> AEQATKSVLFVCLGNICRSPIAEAVFRKLVTDQNISENWVIDSGAVSDWNVGRSPDPRAVSCLRNHGIHTAHKARQITKEDFATFDYILCMDESNLRDLNRKSNQVKTCKAKIELLGSYDPQKQLIIEDPYYGNDS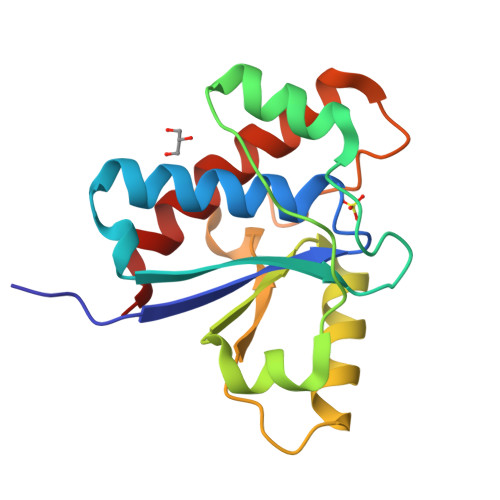DFETVYQQCVRCCRAFLEKAH> GSFTSHQVAGHMYGKILQHPDGTVLKQLQPPPRGPRELEFYNMVYAADCFDGVLLELRKYLPKYYGIWSPPTAPNDLYLKL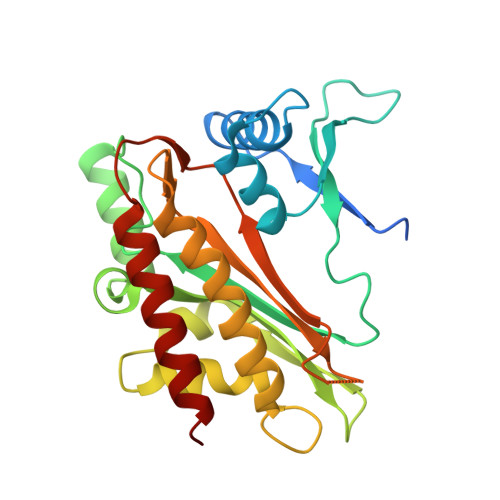EDVTHKFNKPCIMDVKIGQKSYDPFASSEKIQQQVSKYPLMEEIGFLVLGMRVYHVHSDSYETENQHYGRSLTKETIKDGVSRFFHNGYCLRKDAVAASIQKIEKILQWFENQKQLNFYASSLLFVYEGSSQGGSGGEVEVRMIDFAHVFPSNTIDEGYVYGLKHLISVLRSILDN>[24x]MTEYEG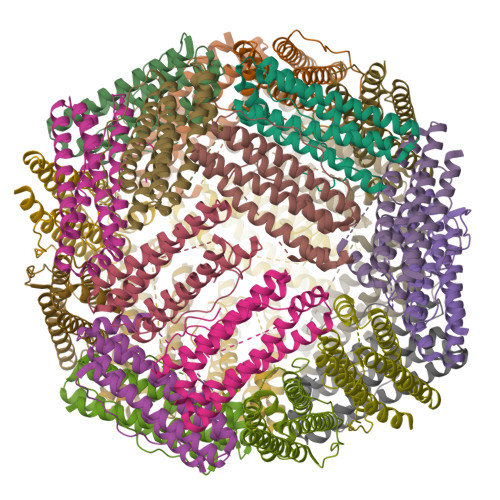PKTKFHALMQEQIHNEFTAAQQYVAIAVYFDSEDLPQLAKHFYSQAVEERNHAMMLVQHLLDRDLRVEIPGVDTVRNQFDRPREALALALDQERTVTDQVGRLTAVARDEGDFLGEQFMQWFLQEQIEEVALMATLVRVADRAGANLFELENFVAREVDVAPAASGAPHAAGGRL> MAVQLHVWGPAFGLPSIDAECLAAIAYLAQTLGSADYQLIQSSPSAVPTQHLPTLYDSRTSTWIGGFTSITAHLHTHPPPTFQSAPQPTDGSSST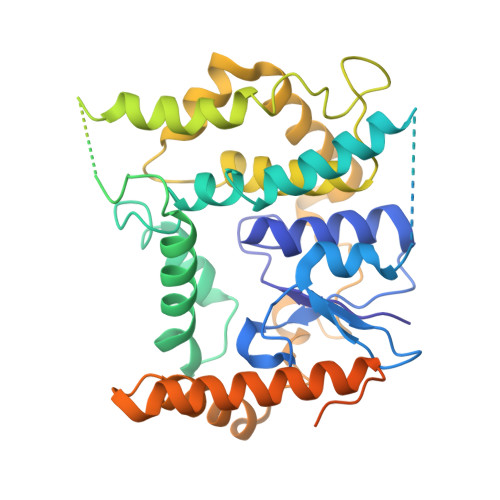TTTTTTTTTAASATADGTAYTAFLSAHAAPLLALSLYVSSANYGAATRPAYSAVLPLPLPWTEPPAVRAAMARRAAHLGLSSLDADAAAERARAEERRAAADGWVAVPPHATAGRAAGGGGGGGGGGGKGGGVAAVLTPEQKSRIRLEEAAREVLDVLAEVDWAAGGGGRQVAAEVRCLAFGYLALMLLPDVPRPWLREIMEGRYPALCTFVRDFRARVFPQGGKLLPWADGGAQASASASASASAVALRFVRAVMAEVPLVGEWWSRWWTARKKREVLASKGAKPAPSNDLLLLLGAGLGLTVVGAGVFFYRGLPPFGEAVQVWRKPVVGLSSFGAAGAMFSGALYGLD>[2x]MTREELLRENIELAKEHIEIMREILELLQKMEELLEKARGADEDVAKTIKELLRRLKEIIERNQRIAKEHEYIARERS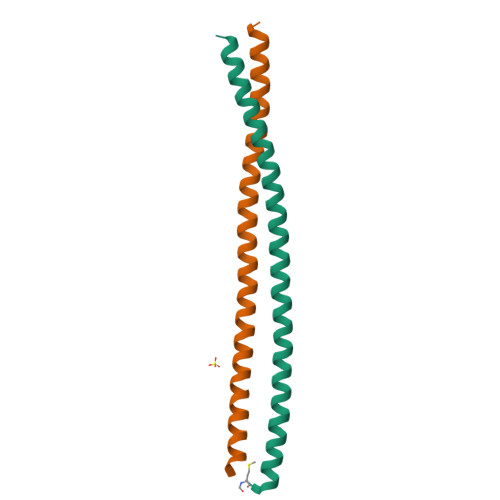;>[2x]GTERKLLERSRRLQEESKRLLDEMAEIMRRIKKLLKKARGADEKVLDELRKIIERIRELLDRSRKIHERSEEIAYKEE>MSDGKKHVVIIGGGITGLAAAFYMEKEIKEKNLPLELTLVEASPRVGGKIQTVKKDGYIIERGPDSFLERKKSAPQLVKDLGLEHLLVNNATGQSYVLVNRTLHPMPKGAVMGIPTKIAPFVSTGLFSLSGKARAAMDFILPASKTKDDQSLGEFFRRRVGDEVVENLIEPLLSGIYAGDIDKLSLMSTFPQFYQTEQKHRSLILGMKKTRPQGSGQQLTAKKQGQFQTLSTGLQTLVEEIEKQLKLTKVYKGTKVTKLSHSGSCYSLELDNGVTLDADSVIVTAPHKAAAGMLSELPAISHLKNMHSTSVANVALGFPEGSVQMEHEGTGFVISRNSDFAITACTWTNKKWPHAAPEGKTLLRAYVGKAGDESIVDLSDNDIINIVLEDLKKVMNINGEPEMTCVTRWHESMPQYHVGHKQRIKELREALASAYPGVYMTGASFEGVGIPDCID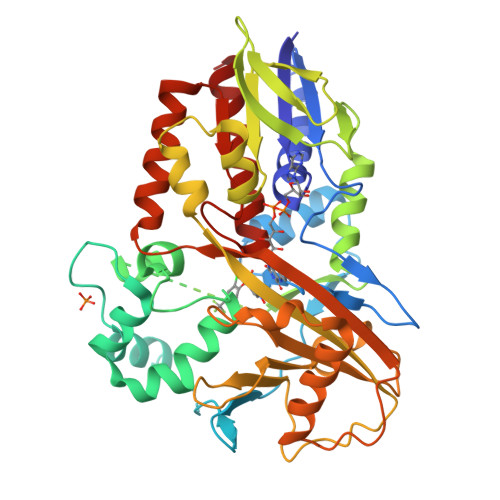QGKAAVSDALTYLFS[2x]> RSSHHHHHHGEFDDPIRPPLKVARSPRPGQCQDVVQDVPNVDVQMLELYDRMSFKDIDGGVWKQGWNIKYDPLKYNAHHKLKVFVVPHSHNDPGWIQTFEEYYQHDTKHILSNALRHLHDNPEMKFIWAEISYFARFYHDLGENKKLQMKSIVKNGQLEFVTGGWVMPDEANSHWRNVLLQLTEGQTWLKQFMNVTPTASWAIDPFGHSPTMPYILQKSGFKNMLIQRTHYSVKKELAQQRQLEFLWRQIWDNKGDTALFTHMMPFYSYDIPHTCGPDPKVCCQFDFKRMGSFGLSCPWKVPPRTISDQNVAARSDLLVDQWKKKAELYRTNVLLIPLGDNFRFKQNTEWDVQRVNYERLFEHINSQAHFNVQAQFGTLQEYFDAVHQAERAGQAEFPTLSGDFFTYADRSDNYWSGYYTSRPYHKRMDRVLMHYVRAAEMLSAWHSWDGMARIEERLEQARRELSLFQHHDGITGTAKTHVVVDYEQRMQEALKACQMVMQQSVYRLLTKPSIYSPDFSFSYFTLDDSRWPGSGVEDSRTTIILGEDILPSKHVVMHNTLPHWREQLVDFYVSSPFVSVTDLANNPVEAQVSPVWSWHHDTLTKTIHPQGSTTKYR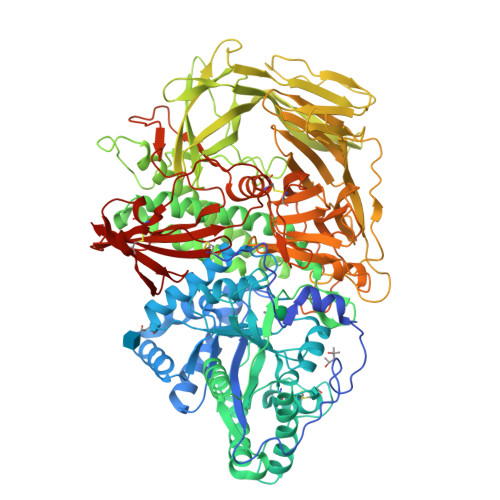IIFKARVPPMGLATYVLTISDSKPEHTSYASNLLLRKNPTSLPLGQYPEDVKFGDPREISLRVGNGPTLAFSEQGLLKSIQLTQDSPHVPVHFKFLKYGVRSHGDRSGAYLFLPNGPASPVELGQPVVLVTKGKLESSVSVGLPSVVHQTIMRGGAPEIRNLVDIGSLDNTEIVMRLETHIDSGDIFYTDLNGLQFIKRRRLDKLPLQANYYPIPSGMFIEDANTRLTLLTGQPLGGSSLASGELEIMQDRRLASDDERGLGQGVLDNKPVLHIYRLVLEKVNNCVRPSKLHPAGYLTSAAHKASQSLLDPLDKFIFAENEWIGAQGQFGGDHPSAREDLDVSVMRRLTKSSAKTQRVGYVLHRTNLMQCGTPEEHTQKLDVCHLLPNVARCERTTLTFLQNLEHLDGMVAPEVCPMETAAYVSSHSS> MTVRKNQATLTADEKRRFVAAVLELKRSGRYDEFVRTHNEFIMSDTDSGERTGHRSPSFLPWHRRFLLDFEQALQSVDSSVTLPYWDWSADRTVRASLWAPDFLGGTGRSTDGRVMDGPFAASTGNWPINVRVDSRTYLRRSLGGSVAELPTRAEVESVLAISAYDLPPYNSASEGFRNHLEGWRGVNLHNRVHVWVGGQMATGVSPNDPVFWLHHAYVDKLWAEWQRRHPDSAYVPTGGTPDVVDLNETMKPWNTVRPADLLDHTAYYTFDALEHHHHHH;> MPEITRRRALTAAAAVAATASAAVT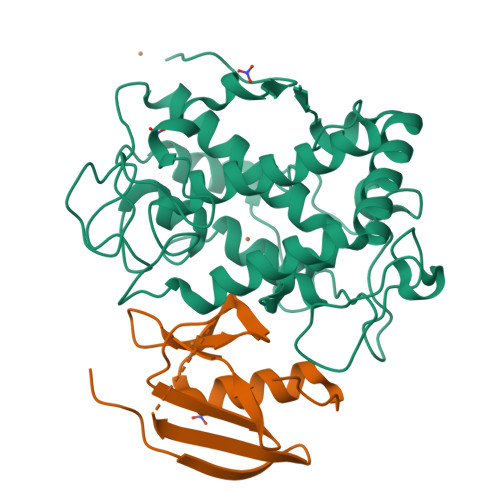LAAPAASAAGHHEPAAPESFDEVYKGRRIQGRPAGGGAHHHEHGGGYEVFVDGVQLHVMRNADGSWISVVSQYDPVPTPRAAARAAVDELQGAPLLPFPANLEHHHHHH>RVCPRILLECKKDSDCLAECVCLEHG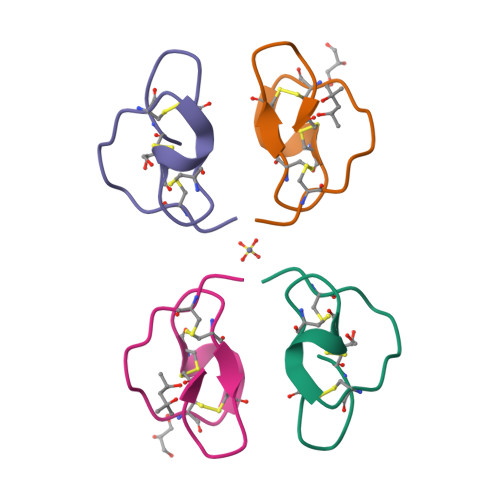YCG[2x]>[6x]MGSSHHHHHHSNMSQEKKVFKTEWAGRSLTIETGQLAKQANGAVLVRYGDTVVLSTATASKEPRDGDFFPLTVNYEEKMYAAGKIPGGFKKREGRPGDEATLTARLIDRPIRPLFPKGYRH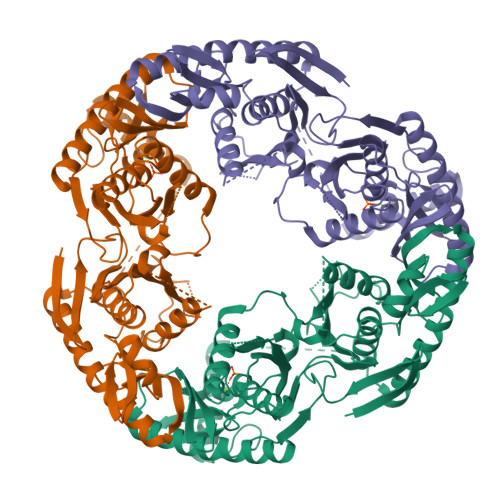DVQIMNIVLSADPDCSPEMAAMIGSSMALSVSDIPFQGPIAGVNVGYIDGKYVINPSVADKEISRLDLEVAGHKDAVNMVEAGASEITESEMLEAIFFGHEEIKRLVAFQQEIIDHIQPIKQEFVPVERDEDLVEKVKSLTEDKGLKDTVLTFDKQQRDENLDALKEEVVGHFLDEEDPENETLVKEVYAILNDLIKEEVRRLIADEKIRPDGRKVDEIRPLESEVGLLPRAHGSGLFTRGQTQALSVLTLGALGDYQLIDGLGPEVEKRFMHHYNFPNFSVGETGPVRAPGRREIGHGALGERALRYIIPDTQDFPYTIRIVSEVLESNGSSSQASICGSTLALMDAGVPIKAPVAGIAMGLVTRDDSYTILTDIQGMEDALGDMDFKVAGTKDGITAIQMDIKIDGLTREVIEEALEQARQGRLAIMDHMLHTIEQPREELSAYAPKVVTMSINPDKIRDVIGPGGKKINEIIDETGVKLDIEQDGTIFIGAVDQAMINRAKEIIEDITREAEVGQVYHAKVKRIEKYGAFVELFPGKDALLHISQISQERINKVEDVLKIGDTIEVKITEIDKQGRVNASHKVLEQSKN>MGLPLMMERSSNNNNVELSRVAVSDTHGEDSPYFAGWKAYDENPYDESHNPSGVIQMGLAENQVSFDLLETYLEKKNPEGSMWGSKGAPGFRENALFQDYHGLKTFRQAMASFMEQIRGGKARFDPDRIVLTAGATAANELLTFILADPNDALLVPTPYYPGFDRDLRWRTGVKIVPIHCDSSNHFQITPEALESAYQTARDANIRVRGVLITNPSNPLGATVQKKVLEDLLDFCVRKNIHLVSDEIYSGSVFHASEFTSVAEIVENIDDVSVKERVHIVYSLSKDLGLPGFRVGTIYSYNDNVVRTARRMSSFT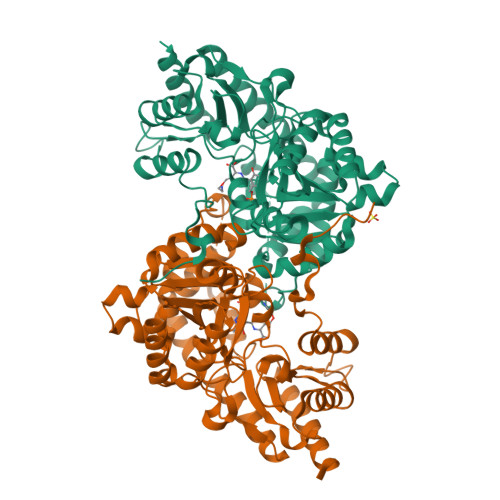LVSSQTQHMLASMLSDEEFTEKYIRINRERLRRRYDTIVEGLKKAGIECLKGNAGLFCWMNLGFLLEKKTKDGELQLWDVILKELNLNISPGSSCHCSEVGWFRVCFANMSENTLEIALKRIHEFMDRRRRF[4x]> MYYFIPSWSGSGKRVWHRDIIPWYRSMQRLEFDDTIHQIRIFHSENLPVKLLLQAYMPHARYFLHRQDIFETEYYSVFDEIQAVESNDMQVLQIKDLEWEDDCEFIYTPFLIIVRRQGQLYAHVEFGVEGFISFIKFFKDDQLEKLNIFDDRGFVSSIVYYEDGQEVCQDYLNPNGDWRIREYLKFENSHVVVNPVFSRDFDKLEYECMPDLILEKLGYYISHNVEEDSRFVVAAQPFTNQGVLDLLPQHSHSILSFFHERNQASNIENLKADLEYADLVLTDRMDFKETLQNYFPLQAEKIHYLSPFDTRLQLGKSQQRHESKIFYQIDLSELLNDYAIFKVLFYVAQHPDTELVIGVYNAWQEGIKQVENKVEELISDYLDLKDFIKKSFKNNQAENPLPENQELEYRFRIRNITDELS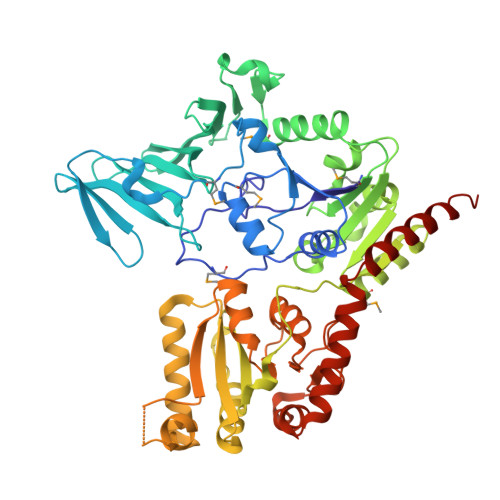LIQELDDTRLIIDLSQQPNLYTQIAGISAGIPQINLVASDYVTHLQNGYILDSISQLAVAADYYLQGLKNWNQALIYSIEKIKLNTGHQVIKRWEKWLKEAIDEKVDKLVPR>GSIYTFNELVVLDYPHKDRALRYLERLRDDTGIKKIMDSHRWTVPLLSEMDPAEHTRHDSKTLGLNH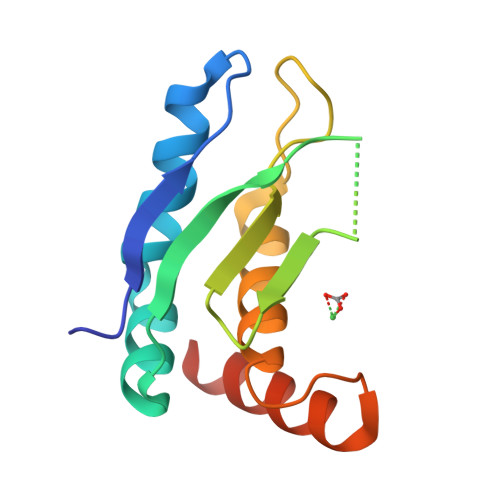NQGAHIELRLRTDRYDGFRDYKTVKSTLIHQLTHNVHGEHDSSFWELFRQLTKEADAADLL[2x]>TGGCCTTAAGG[2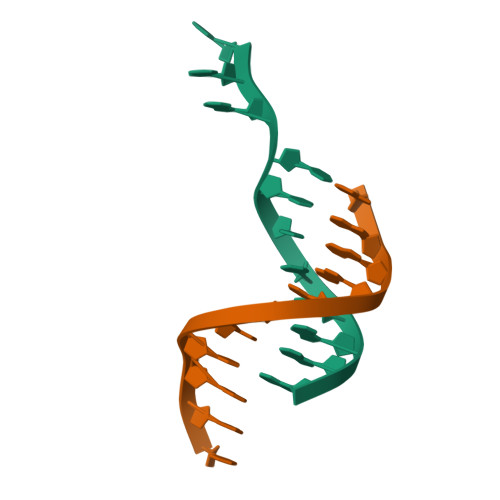x]> GPMVAMFQEDNGTSSVASSPLQVFSTMSLNRPTLLASSSPFHCLKDLKPEERGLYLIHLLLTCANHVASGSLQNANAALEQLSHLASPDGDTMQRIAAYFTEALANRILKSWPGLYKALNATQTRTNNVSEEIHVRRLFFEMFPILKVSYLLTNRAILEAMEGEKMVHVIDLDASEPAQWLALLQAFNSRPEGPPHLRITGVHHQKEVLEQMAHRLIEEAEKLDIPFQFN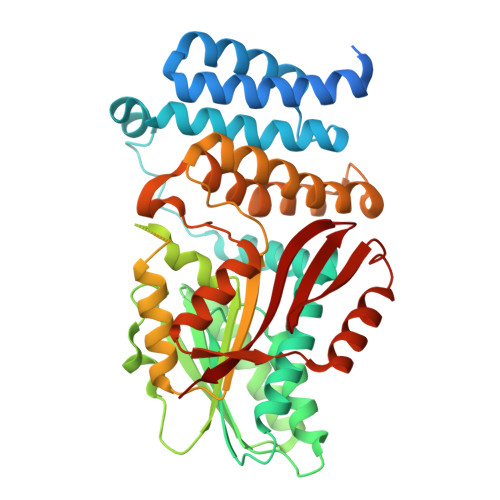PVVSRLDCLNVEQLRVKTGEALAVSSVLQLHTFLASDDDLMRKNCALRFQNNPSGVDLQRVLMMSHGSAAEARENDMSNNNGYSPSGDSASSLPLPSSGRTDSFLNAIWGLSPKVMVVTEQDSDHNGSTLMERLLESLYTYAALFDCLETKVPRTSQDRIKVEKMLFGEEIKNIISCEGFERRERHEKLEKWSQRIDLAGFGNVPLSYYAMLQARRLLQGCGFDGYRIKEESGCAVICWQDRPLYSVSAWRCRK> MAKINELLRESTTTNSNSIGRPNLVALTRATTKLIYSDIVATQRTNQPVAAFYGIKYLNPDNEFTFKTGATYAGEAGYVDREQITELTEESKLTLNKGDLFKYNNIVYKVLEDTPFATIEESDLELALQIAIVLLKVRLFSDA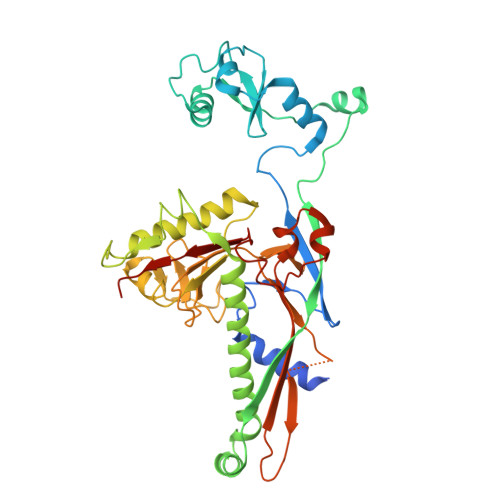ASTSKFESSDSEIADARFQINKWQTAVKSRKLKTGITVELAQDLEANGFDAPNFLEDLLATEMADEINKDILQSLITVSKRYKVTGITDSGFIDLSYASAPEAGRSLYRMVCEMVSHIQKESTYTATFCVASARAAAILAASGWLKHKPEDDKYLSQNAYGFLANGLPLYCDTNSPLDYVIVGVVENIGEKEIVGSIFYAPYTEGLDLDDPEHVGAFKVVVDPESLQPSIGLLVRYALSANPYTVAKDEKEARIIDGGDMDKMAGRSDLSVLLGVKLPKIIIDE> GPHMQKYEYKSDQWKPLNLEEKKRYDREFLLGFQFIFASMQKPEG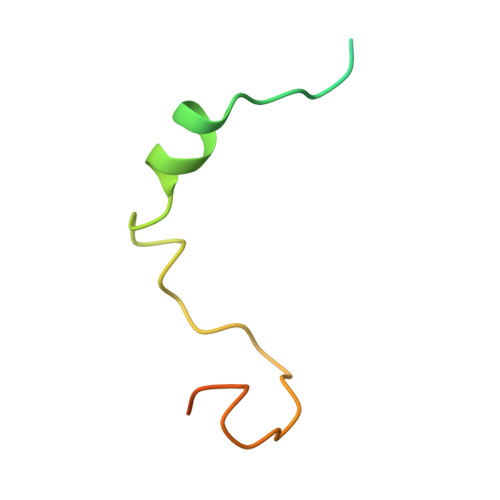LPHISDVVLDKANKTPLRPLD>MFTGSIVAIVTPMDEKGNVCRASLKKLIDYHVASGTSAIVSVGTTGESATLNHDEHADVVMMTLDLADGRIPVIAGTGANATAEAISLTQRFNDSGIVGCLTVTPYYNRPSQEGLYQHFKAIAEHTDLPQILYNVPSRTGCDLLPETVGRLAKVKNIIGIKEATGNLT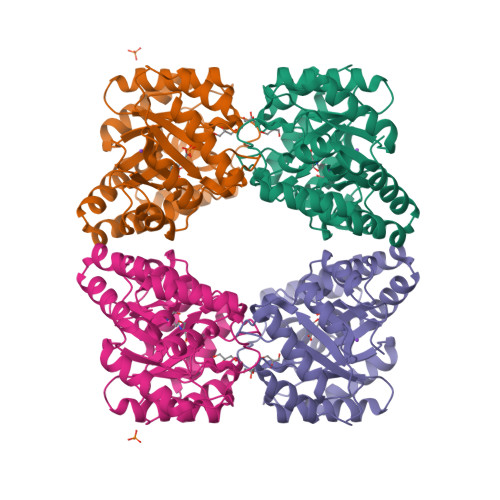RVNQIKELVSDDFVLLSGDDASALDFMQLGGHGVISVTANVAARDMAQMCKLAAEGHFAEARVINQRLMPLHNKLFVEPNPIPVKWACKELGLVATDTLRLPMTPITDSGRETVRAALKHAGLL[2x]> LRPKLSEEQQRIIAILLDAHHKTYDPTYSDFCQFRPPVRVNDGGGSVTLELSQLSMLPHLADLVSYSIQKVIGFAKMIPGFRDLTSEDQIVLLKSSAIEVIMLRSNESFTMDDMSWTCGNQDYKYRVSDVTKAGQSLELIEPLIK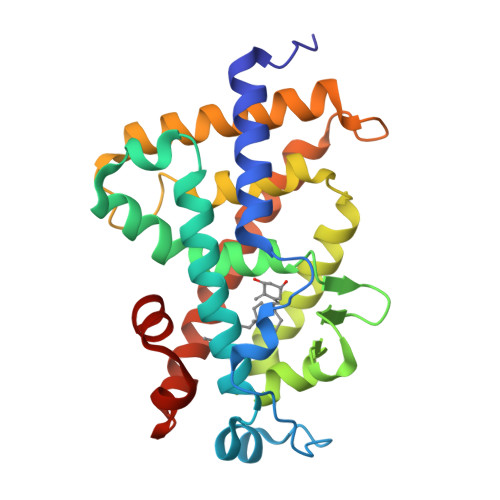FQVGLKKLNLHEEEHVLLMAICIVSPDRPGVQDAALIEAIQDRLSNTLQTYIRCRHPPPGSHLLYAKMIQKLADLRSLNEEHSKQYRCLSFQPECSMKLTPLVLEVFG> MAVPFVEDWDLVQTLGEGAYGEVQLAVNRVTEEAVAVKIVDMKRAVDCPENIKKEICINKMLNHENVVKFYGHRREGNIQYLFLEYCSGGELFDRIEPDIGMPEPDAQRFFHQLMAGVVYLHGIGITHRDIKPENLLLDERDNLKISDFGLATVFRYNNRERLLNKMCGTLPYVAPELLKRREFHAEPVDVWSCGIVLTAMLA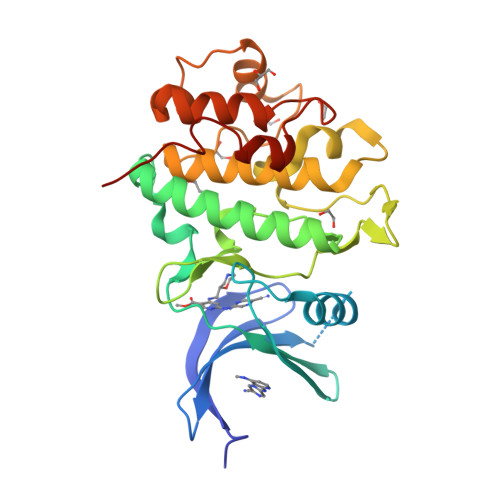GELPWDQPSDSCQEYSDWKEKKTYLNPWKKIDSAPLALLHKILVENPSARITIPDIKKDRWYNKPLKKGA> MKPDETPMFDPSLLKEVDWSQNTATFSPAISPTHPGEGLVLRPLCTADLNRGFFKVLGQLTETGVVSPEQFMKSFEHMKKSGDYYVTVVEDVTLGQIVATATLIIEHKFIHSCAKRGRVEDVVVSDECRGKQLGKLLLSTLTLLSKKLNCYKITLECLPQNVGFYKKFGYTVSEE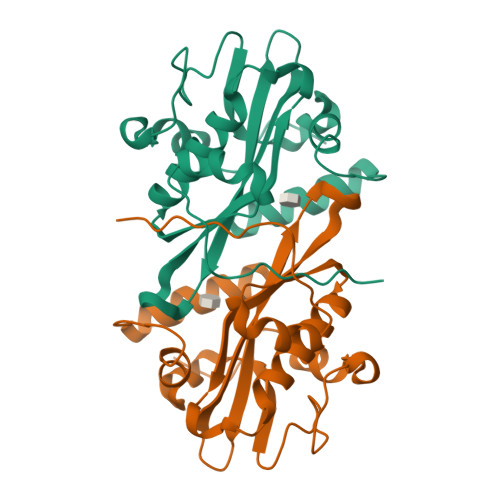NYMCRRFLK>SIDEVGALSKFAASLADQMRAGSNSLDRDVQSLFGVWKGSAADAYRSGWDEMQDGATKVWNALTDIASTLGSNAAAFHAQETSTASSITSTQAD[6x];>[6x]MAAHVESEFSFDLDHIEQVTSRARGFKEFVTENLDQLESRAQKLVQSGQWAGAAAAAYSQAHKEWMDAARELVEGLSQMEEAARTAHGAYSEAQEANLRMARG

Of particular interest are the Esx complexes which are dimers of two subunits (ESAT-6, early secreted antigen of 6 kDa; and CFP-10, culture filtrate protein of 10 kDa) and which are secreted across the cytoplasmic membrane by Type VII secretion (T7S) systems. Mycobacterial ESX secretion systems have been shown to be involved in a variety of physiological processes including conjugation in a non-pathogenic mycobacterium, iron and/or zinc acquisition by both pathogenic and non-pathogenic mycobacterial species, and virulence of pathogenic mycobacteria. The overall architecture of the complexes is similar to known Esx structures in that each heterodimer forms a four helix bundle with the CFP-10 and ESAT-6 subunit homologs each contributing an α-helical hairpin to the complex. The subunit interfaces in the four-helix bundles of the Esx complexes are similar to those of the previously determined Esx complex structures in that the intermolecular interface between the CFP-10 and ESAT-6 subunits is largely hydrophobic.

Using this expression approach we expressed and purified six Esx complexes and determined the crystal structures of M. abscessus EsxEF (EsxEFma), encoded by the MAB_3112 and MAB_3113 genes, M. smegmatis EsxGH (EsxGHms), encoded by the MSMEG_0620 and MSMEG_0621 genes, and M. tuberculosis EsxOP (EsxOPmt), encoded by the Rv2346c and Rv2347c genes, at resolutions of 1.96 Å, 2.70 Å, and 2.55 Å, respectively. Three additional Esx complexes (EsxGHma, EsxEFma, and EsxTUma) from M. abscessus, a fast-growing pathogen, were cloned into pMAPLe4, an expression vector similar to pMAPLe3 with the exception that the MBP moiety is cleaved from the CFP-10 passenger by TVMV protease leaving a TEV protease cleavable His6 tag on the N-terminus of the CFP-10 subunit. The substitution of an N-terminal cleavable tag on the CFP-10 subunit in lieu of the C-terminal His6 tag on the ESAT-6 subunit was deemed to be more amenable to generating a well ordered crystal lattice as the number of potentially disordered amino acid residues is reduced. A crude low resolution model of the SeMet-labeled EsxEFma complex was used to obtain a molecular replacement solution for a high resolution (1.96 Å) EsxEFma native dataset and a second crystal form of EsxOPmt, solved by molecular replacement using the EsxOPmt model from form I, at 2.55 Å was also obtained. The asymmetric units for the EsxEFma crystal forms have a single complex in the asymmetric unit for the SeMet-labeled protein and six complexes in the asymmetric unit of the native protein crystal form while the EsxGHms and EsxOPmt (both crystal forms) contain two heterodimeric complexes. The WXG-containing loops are well ordered in the EsxGHms complexes and in most of the EsxEFma complexes but the majority of the connecting loops are disordered in the EsxOPmt subunit structures.> DY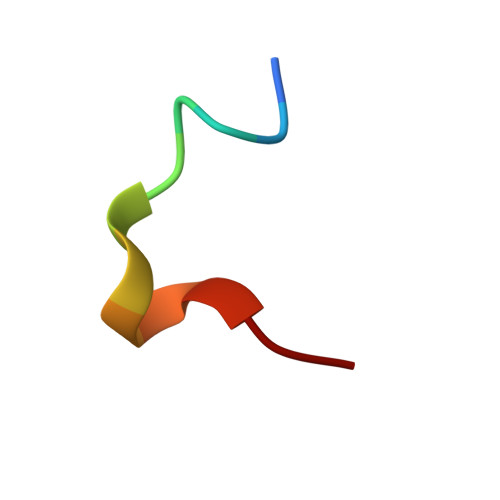LDIPAFLRKQ Protoglobin (Pgb) is a recently discovered haem-protein with distinct structural and functional features that make it unique within the globin superfamily. The MaPgb* structure can be considered as an expanded version of the 3/3 helical sandwich typical of “classical” globins (i.e. Mb), with an additional N-terminal extension, built by a 20-residue loop, followed by the Z-helix, which precedes the globin-fold conserved A-helix. Residues belonging to the Z-helix contribute to formation of the Pgb homodimer, which is centered on the intermolecular four-helix bundle built by the G- and H-helices of the two subunits. Thus, in Pgb the access of diatomic ligands, such as O2, CO, and NO, to the haem is granted by two orthogonal apolar tunnels that reach the haem distal region from entry sites at the B/G and B/E helix interfaces.

To verify whether molecules larger than azide could be coordinated to the MaPgb* haem-Fe(III) atom, imidazole binding was tested on the crystalline protein. The structure of the MaPgb*(III)-imidazole complex was solved at 1.38 Å resolution (one MaPgb* molecule in the asymmetric unit) and refined to final R-factor of 15.9% and R-free of 19.8%. The structure of MaPgb*(III)-imidazole is well superimposable in its backbone to that of the MaPgb*(III)-cyanide complex (rms deviation values calculated for 190 Cα atom pairs ranging between 0.41 Å and 0.45 Å, depending on the superimposed subunits), and their dimeric quaternary structure are identical. The azimuthal orientation of the haem-Fe(III)-bound imidazole is staggered relative to the haem pyrrole nitrogen atoms (lying at about 15° from a line connecting the methinic CHA-CHC atoms), with a haem-Fe(III) coordination bond of 1.97 Å. The haem-Fe(III)-bound imidazole was refined in a double conformation (occupancy of 0.5 each) with the imidazole N3 atom pointing alternatively towards the Tyr(B10)61 OH group (2.69 Å distance), and the Nε1 atom of Trp(B9)60 (2.64 Å distance). Additional stabilizing interactions are provided by several van der Waals contacts involving the hydrophobic MaPgb*(III) haem distal site residues, such as Val(B13)64, Phe(CD1)74, Val(E7)89, Phe(E11)93, and Phe(G7)145, surrounding the haem-Fe(III)-bound imidazole. Overall, the haem distal site structure of the MaPgb*(III)-imidazole complex superimposes well with that of MaPgb*(III)-cyanide. Small differences occur in the position of the Tyr(61)B10 OH group (a shift of 0.75 Å), and the rotation of the Phe(93)E11 side chain around the Cβ-Cγ bond (of ∼13°). Thus, the ligand sensing mechanism of the Phe(93)E11 is preserved and the Trp(B9)60 side chain is properly oriented in the haem distal site cavity to stabilize the haem-Fe(III)-bound imidazole and to shut tunnel 1.

> MSVEKIPGYTYGETENRAPFNLEDLKLLKEAVMFTAEDEEYIQKAGEVLEDQVEEILDTWYGFVGSHPHLLYYFTSPDGTPNEKYLAAVRKRFSRWILDTSNRSYDQAWLDYQYEIGLRHHRTKKNQTDNVESVPNIGYRYLVAFIYPITATMKPFLARKGHTPEEVEKMYQAWFKATTLQVALWSYPYVKYGDF> GSHMVRKNPKSDKFKVKRFHHIEFWCGDATNVARRFSWGLGMRFSAKSDLSTGNMVHASYLLTSGDLRFLFTAPYSPSLSAGEIKPTTTASIPSFDHGSCRSFFSS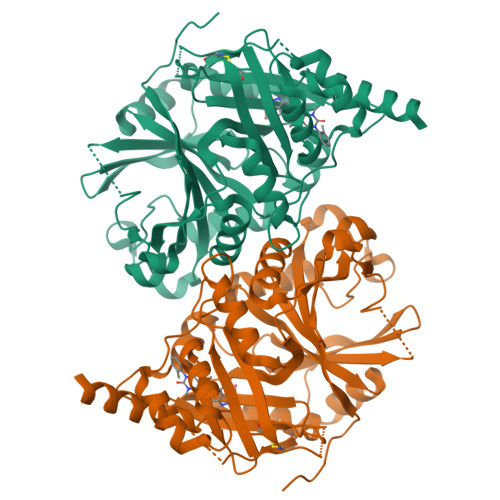HGLGVRAVAIEVEDAESAFSISVANGAIPSSPPIVLNEAVTIAEVKLYGDVVLRYVSYKAEDTEKSEFLPGFERVEDASSFPLDYGIRRLDHAVGNVPELGPALTYVAGFTGFHQFAEFTADDVGTAESGLNSAVLASNDEMVLLPINEPVHGTKRKSQIQTYLEHNEGAGLQHLALMSEDIFRTLREMRKRSSIGGFDFMPSPPPTYYQNLKKRVGDVLSDDQIKECEELGILVDRDDQGTLLQIFTKPLGDRPTIFIEIIQRVGCMMKDEEGKAYQSGGCGGFGKGNFSELFKSIEEYEKTL>GSEGAATMSHTILLVQPTKRPEGRTYADYESVNECMEGVCKMYEEHLKRMNPNSPSITYDISQLFDFIDDLADLSCLVYRADTQTYQPYNKDWIKEKIYVLLRRQA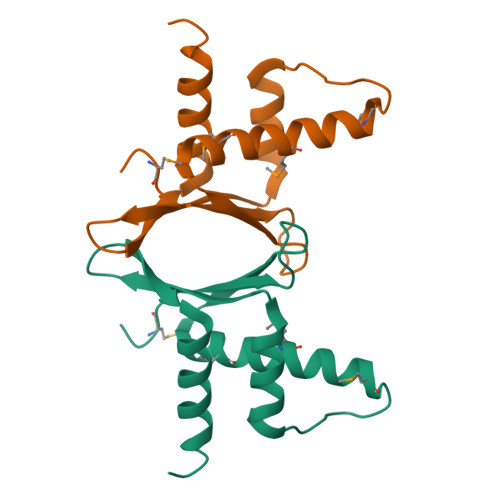QQAGK[3x]> MWRVCARRAQNVAPWAGLEARWTALQEVPGTPRVTSRSGPAPARRNSVTTGYGGVRALCGWTPSSGATPRNRLLLQLLGSPGRRYYSLPPHQKVPLPSLSPTMQAGTIARWEKKEGDKINEGDLIAEVETDKATVGFESLEECYMAKILVAEGT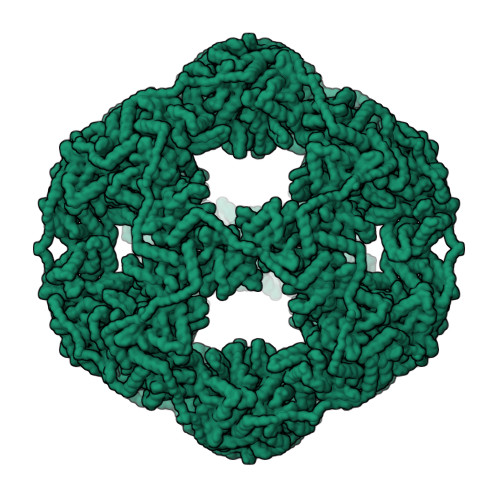RDVPIGAIICITVGKPEDIEAFKNYTLDSSAAPTPQAAPAPTPAATASPPTPSAQAPGSSYPPHMQVLLPALSPTMTMGTVQRWEKKVGEKLSEGDLLAEIETDKATIGFEVQEEGYLAKILVPEGTRDVPLGTPLCIIVEKEADISAFADYRPTEVTDLKPQVPPPTPPPVAAVPPTPQPLAPTPSAPCPATPAGPKGRVFVSPLAKKLAVEKGIDLTQVKGTGPDGRITKKDIDSFVPSKVAPAPAAVVPPTGPGMAPVPTGVFTDIPISNIRRVIAQRLMQSKQTIPHYYLSIDVNMGEVLLVRKELNKILEGRSKISVNDFIIKASALACLKVPEANSSWMDTVIRQNHVVDVSVAVSTPAGLITPIVFNAHIKGVETIANDVVSLATKAREGKLQPHEFQGGTFTISNLGMFGIKNFSAIINPPQACILAIGASEDKLVPADNEKGFDVASMMSVTLSCDHRVVDGAVGAQWLAEFRKYLEKPITMLL>[8x]MSQQPGVLPENMKRYMGRDAQRMNILAGRIIAETVRSTLGPKGMDKMLVDDLGDVVVTNDGVTILREMSVEHPAAKMLIEVAKTQEKEVGDGTTTAVVVAGELLRKAEELLDQNVHPTIVVKGYQAAAQKAQELLKTIACEVGAQDKEILTKIAMTSITGKGAEKAKEKLAEIIVEAVSAVVDDEGKVDKDLIKIEKKSGASIDDTELIKGVLVDKERVSAQMPKKVTDAKIALLNCAIEIKETETDAEIRITDPAKLMEFIEQ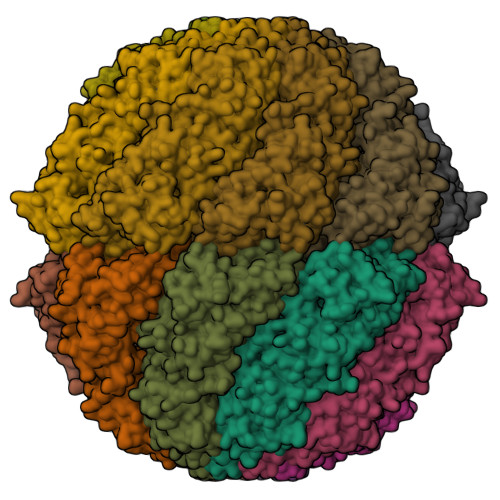EEKMLKDMVAEIKASGANVLFCQKGIDDLAQHYLAKEGIVAARRVKKSDMEKLAKATGANVITNIKDLSAQDLGDAGLVEERKISGDSMIFVEECKHPKAVTMLIRGTTEHVIEEVARAVDDAVGVVGCTIEDGRIVSGGGSTEVELSMKLREYAEGISGREQLAVRAFADALEVIPRTLAENAGLDAIEILVKVRAAHASNGNKCAGLNVFTGAVEDMCENGVVEPLRVKTQAIQSAAESTEMLLRIDDVIAAEKLRGAPDMGDMGGMPGMGGMPGMM> GPMPVFHTRTIESILEPVAQQISHLVIMHEEGEVDGKAIPDLTAPVAAV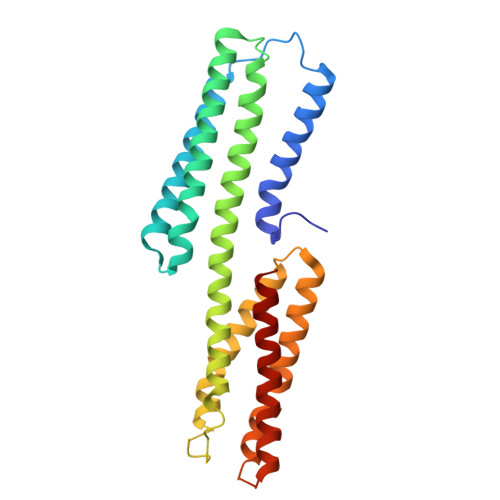QAAVSNLVRVGKETVQTTEDQILKRDMPPAFIKVENACTKLVQAAQMLQSDPYSVPARDYLIDGSRGILSGTSDLLLTFDEAEVRKIIRVCKGILEYLTVAEVVETMEDLVTYTKNLGPGMTKMAKMIDERQQELTHQEHRVMLVNSMNTVKELLPVLISAMKIFVTTKNSKNQGIEEALKNRNFTVEKMSAEINEIIRVLQL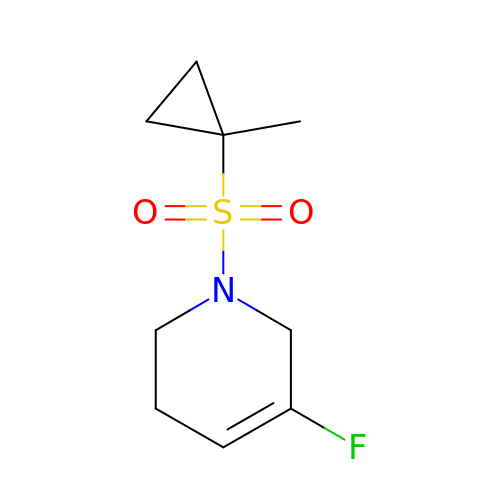5-fluoro-1-(1-methylcyclopropane-1-sulfonyl)-1,2,3,6-tetrahydropyridine | C9 H14 F N O2 S | USHLSOPQTSXCNW-UHFFFAOYSA-N> SCPVNWVEHQDSCYWFSHSGMSWAEAEKYCQLKNAHLVVINSREEQNFVQKYLGSAYTWMGLSDPEGAWKWVDG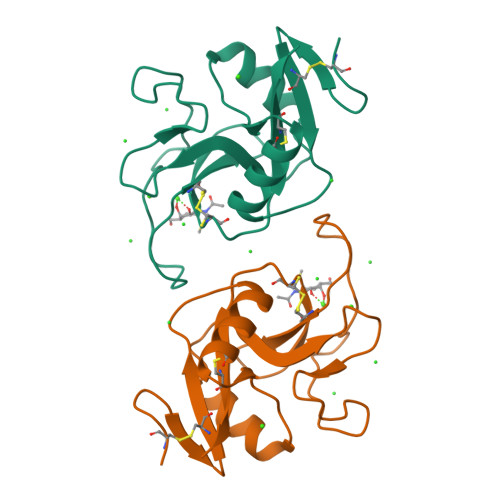TDYATGFQNWKPGQPDDWQGHGLGGGEDCAHFHPDGRWNDDVCQRPYHWVCEAGL> MAMF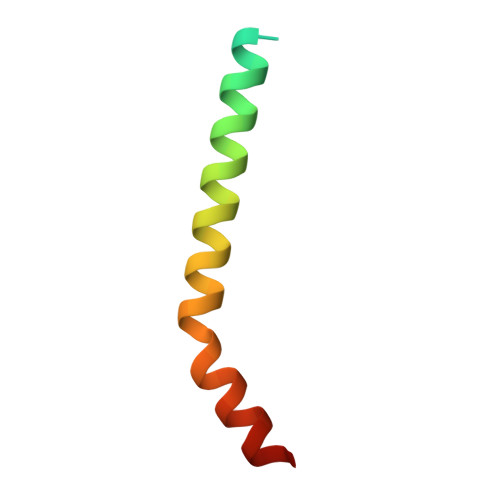GLPQQEVSEEEKRAHQEQTEKTLKQAAYVAAFLWVSPMIWHLVKKQWK>MKIAVMTDSTSYLSQDLIDKYNIQIAPLSVTFDDGKNFTESNEIAIEEFYNKMASSQTIPTTSQPAIGEWITKYEMLRDQGYTDIIVICLSSGISGSYQSSYQAGEMVEGVNVHAFDSKLAAMIEGCYVLRAIEMVEEGYEPQQIIDDLTNMREHTGAYLIVDDLKNLQKSGRITGAQAWVGTLLKMKPVLKFEDGKIIPEEKVRTKKRAIQTLEKKVLDIVKDFEEVTLFVINGDHFEDGQALYKKLQDDCPSA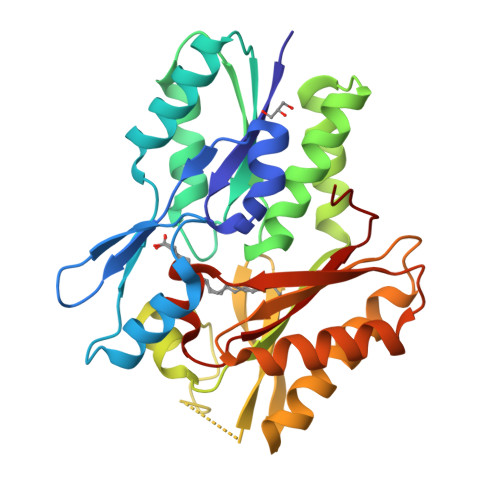YQVAYSETGPVVAAHLGSGGLGLGYVGRKIRLT[2x]>[2x]MASFQSFGIPGQLEVIKKALDHVRVGVVITDPALEDNPIVYVNQGFVQMTGYETEEILGKNCRFLQGKHTDPAEVDNIRTALQNKEPVTVQIQNYKKDGTMFWNELNIDPMEIEDKTYFVGIQNDITEHQQTQARLQELQSELVHVSRLSAMGEMASALAH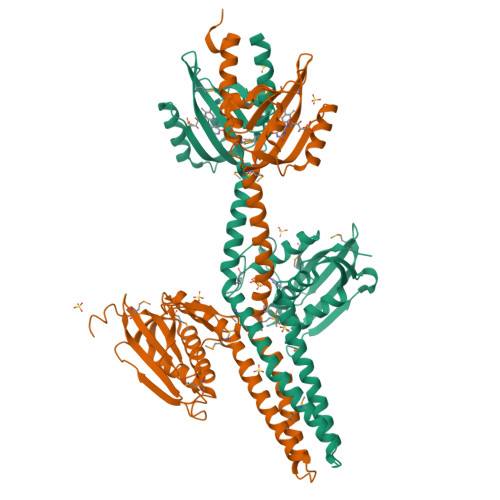ELNQPLAAISNYMKGSRRLLAGSSDPNTPKVESALDRAAEQALRAGQIIRRLRDFVARGESEKRVESLSKLIEEAGALGLAGAREQNVQLRFSLDPGADLVLADRVQIQQVLVNLFRNALEAMAQSQRRELVVTNTPAADDMIEVEVSDTGSGFQDDVIPNLFQTFFTTKDTGMGVGLSISRSIIEAHGGRMWAESNASGGATFRFTLPAADENLEHHHHHHHH>NPEETTAPIMTQGSLYNDSLSTNDFKSILLGSTPLDIAP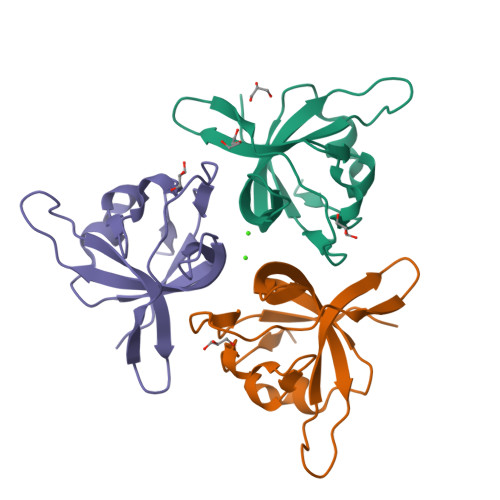DGAVFQLDRPLSIDYSLGTGDVDRAVYWHLKKFAGNAGTPAGWFRWGIWDNFNKTFTDGVAYYSDEQPRQILLPVGTVCTRVDSEN[3x]>[7x]ADSDINIKTGTTDIGSNTTVKTGDLVTYDKENGMHKKVFYSFIDDKNHNKKLLVIRTKGTIAGQYRVYSEEGANKSGLAWPSAFKVQLQLPDNEVAQISD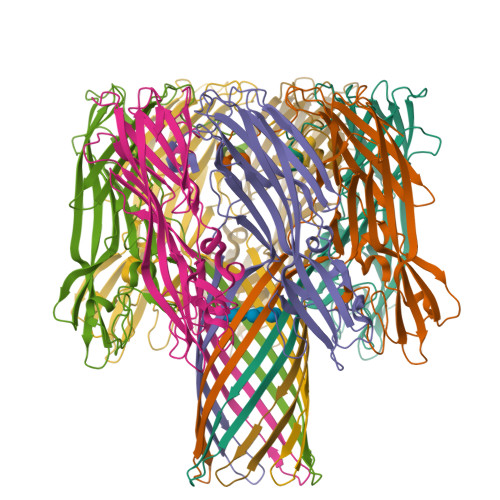YYPRNSIDTKEYNSTLTYGFNGNVTGDDTGKIGGLIGANVSIGHTLKYVQPDFKTILESPTDKKVGWKVIFNNMVNQNWGPYDRDSWNPVYGNQLFMKTRNGSMKAADNFLDPNKASSLLSSGFSPDFATVITMDRKASKQQTNIDVIYERVRDDYQLHWTSTNWKGTNTKDKWTDRSSERYKIDWEKEEMTN N-BENZYLOXYCARBONYL-ALA-PRO-3-AMINO-4-PHENYL-BUTAN-2-OL | C26 H33 N3 O5 | 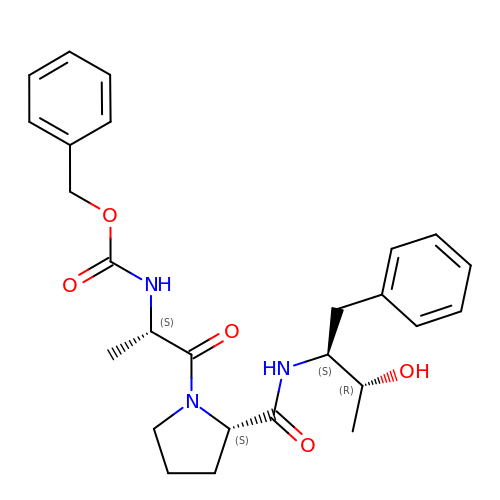MACLRJNEKXUAJK-YDLSIGKMSA-N> MHHHHHHQQIMKGNFSSFMQKEIFEQPESVVNTMRGRVNFDDYTVNLGGLKDHIKEIQRCRRLILIACGTSYHAGVAT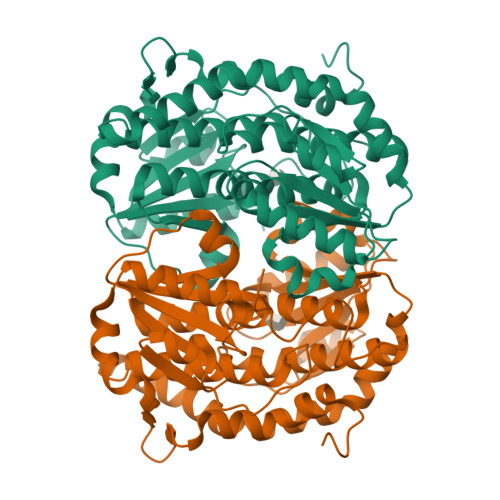RQVLEELTELPVMVELASDFLDRNTPVFRDDVCFFLSQSGETADTLMGLRYCKERGALTVGITNTVGSSISRETDCGVHINAGPEIGVASTKAYTSQFVSLVMFALMMCDDRISMQERRKEIMLGLKRLPDLIKEVLSMDDEIQKLATELYHQKSVLIMGRGYHYATCLEGALKIKEITYMHSEGILAGELKHGPLALVDKLMPVIMIIMRDHTYAKCQNALQQVVARQGRPVVICDKEDTETIKNTKRTIKVPHSVDCLQGILSVIPLQLLAFHLAVLRGYDVDFPRNLAKSVTVE> MPENVAPRSGATAGAAGGRGKGAYQDRDKPAQIRFSNISAAKAVADAIRTSLGPKGMDKMIQDGKGDVTITNDGATILKQMQVLHPAARMLVELSKAQDIEAGDGTTSVVIIAGSLLDSCTKLLQKGIHPTIISESFQKALEKGIEILTDMSRPVELSDRETLLNSATTSLNSKVVSQYSSLLSPMSVNAVMKVIDPATATSVDLRDIKIVKKLGGTIDDCELVEGLVLTQKVSNSGITRVEKAKIGLIQFCLSAPKTDMDNQIVVSDYAQMDRVLREERAYILNLVKQIKKTGCNVLLIQKSILRDALSDLALHFLNKMKIMVIKDIEREDIEFICKTIGTKPVAHIDQFTADMLGSAELAEEVNLNGSGKLLKITGCASPGKTVTIVVRGSNKLVIEEAERSIHDALCVIRCLVKKRALIAGGGAPEIELALRLTEYSRTLSGMESYCVRAFADAMEVIPSTLAENAGLNPISTVTELRNRHAQGEKTAGINVRKGGISNILEELVVQPLLVSVSALTLATETVRSILKIDDVVNTR;> MQDPNADTEWNDILRKKGILPPKESLKELEEEAEEEQRILQQSVVKTYEDMTLEELEDHEDEFNEEDERAIEMYRRRRLAEWKATKLKNKFGEVLEISGKDYVQEVTKAGEGLWVILHLYKQGIPLCALINQHLSGLARKFPDVKFIKAISTTCIPNYPDRNLPTIFVYLEGDIKAQFIGPLVFGGMNLTRDELEWKLSESGAIMTDLEENPKKPIEDVLLSSVRRSVLMKRDSDSEGD

ATP-dependent chaperonin TRiC/CCT partners with cochaperones prefoldin (PFD) and phosducin-like proteins (PhLPs) to facilitate folding of essential eukaryotic proteins. The ring-shaped chaperonin TCP-1 ring complex (TRiC, also called CCT) is a ~1 MDa hetero-oligomeric complex that has a double-chamber architecture, with each octameric ring formed by subunits CCT1-81–3. TRiC-mediated protein folding depends on an ATP-driven conformational cycle, which regulates the opening and closing of a built-in lid over the central chamber of each ring.

However, we could not detect any density attributable to the NTD. We, therefore, performed focused 3D classification on each CCT subunit. This analysis resolved an extended helical density that can be attributed to helix 3 (H3) of the NTD of PhLP2A adopting two different orientations associated with either the apical domain of CCT3 or CCT4. Notably, only the apical domains of CCT3 and CCT4 were predicted to form a dimeric complex with H3 of PhLP2A with good prediction scores, in agreement with our cryoEM density maps. The NTD of PhLP2A can adopt two different orientations, whereby H3 of the NTD contacts the apical regions of either CCT3 or CCT4. While the NTD is mostly negatively charged, H3 has a unique positively charged patch (residue 75–78), which displays a high degree of complementary to the negatively charged apical domains of CCT3 and CCT4 (Fig. 2a(i, ii), b). The charged H3 residues in PhLP2A that contact CCT4 are also highly conserved. In the open state, the PhLP2A NTD adopts an H3 extended conformation to apical domains either CCT3 or 4.>SNAKKEPACFSTVIPGWFSEMSPMWPGEAHSLKVEKVLFQGKSDYQDVIVFQSATYGKVLVLDGVIQLTERDECAYQEMITHLPLCSIPNPKKVLVIGGGDGGVLREVARHASIEQIDMCEIDKMVVDVSKQFFPDVAIGYEDPRVNLVIGDGVAFLKNAAEGSYDAVIVDSSDPIGPAKELFEKPFFQSVARALRPGGVVCTQAESL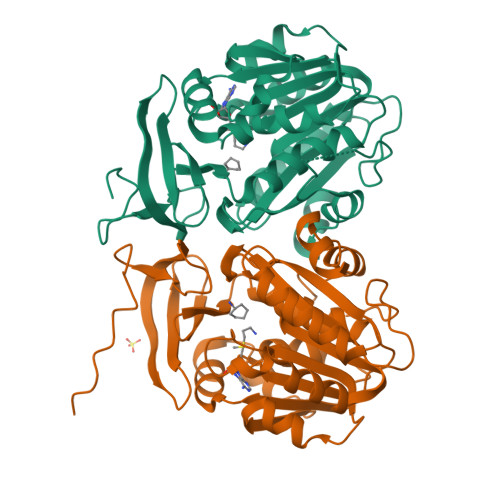WLHMDIIEDIVSNCREIFKGSVNYAWTSVPTYPSGVIGFMLCSTEGPDVDFKHPLNPIDESSSKSNGPLKFYNAEIHSAAFCLPSFAKKVIESKAN[8x]2-[(2S,3R,4R,5R)-5-(hydroxymethyl)-3,4-bis(oxidanyl)-1-pentyl-pyrrolidin-2-yl]-N-methyl-ethanamide 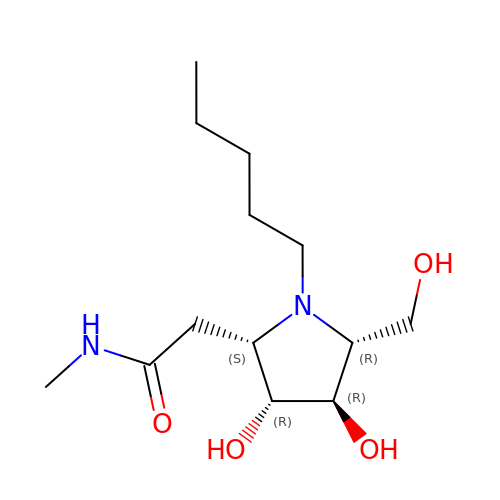| C13 H26 N2 O4 | NZYWNYJYZSBEBH-XKAARJIMSA-N> EFMKVLVIGNGGREHALAWKAAQSPLVETVFVAPGNAGTALEPALQNVAIGVTDIPALLDFAQNEKIDLTIVGPEAPLVKGVVDTFRAAGLKIFGPTAGAAQLEGSKAFTKDFLARHKIPTAEYQNFTEVEPALAYLREKGAPIVIKADGLAAGKGVIVAMTLEEAEAAVHDMLAGNAFGDAGHRIVIEEFLDGEEASFIVMVDGEHVLPMATSQDHKRVGDKDTGPNTGGMGAYSPAPVVTDDVHQRTMERIIWPTVKGMAAEGNTYTGFL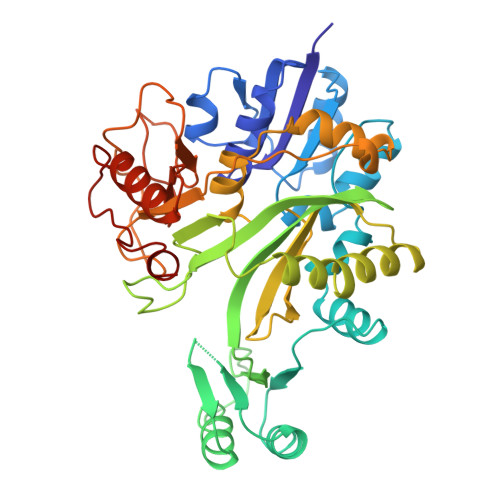YAGLMIDKQGNPKVIEFNCRFGDLETQPIMLRMKSDLVELCLAACESKLDEKTSEWDERASLGVVMAAGGYPGDYRTGDVIHGLPLEEVAGGKVFHAGTKLADDEQVVTNGGRVLCVTALGHTVAEAQKRAYALMTDIHWDDCFCRKDIGWRAIEREQN>ACYCRIPACIAG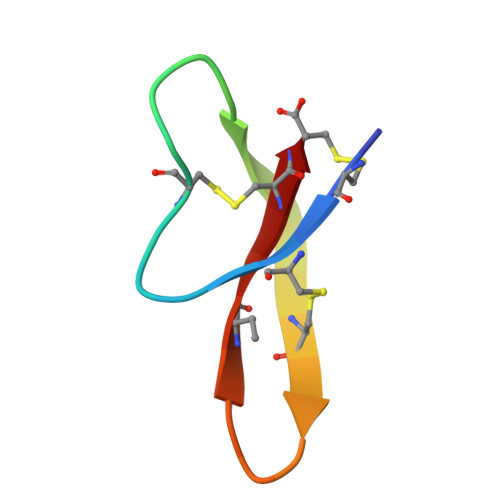ERRYGTCIYQGRLAAFCC[2x]> MNNDSTDKTTVSGYIS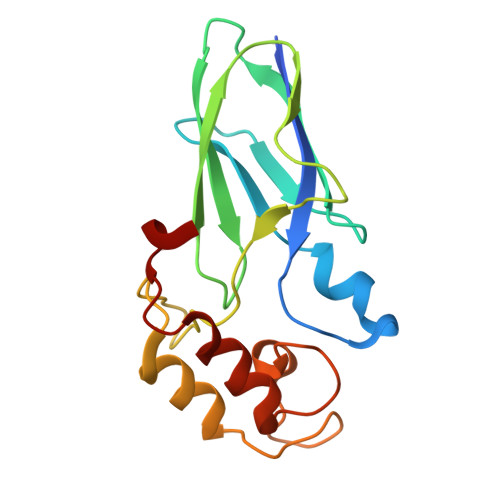VDFDYPPESESKIKSGFNVKVAGTELSTKTDEKGYFEISGIPGDMREFTLEISKRNYLKRNVTVNGTGKLVVSTEDNPLILWAGDVERKGVQDNAINMVDVMEISKVFGTRAGDEEYVAELDLNMDGAINLFDIAIVIRHFNALPSRY> HMSLKSAVKTVLTNSLRSVADGGDWKVLVVDKPALRMISECARMSEILDLGVTVVEDVSKQRKVLPQFHGVYFIEPTEENLDYVIRDFADRTPTYEAAHLFFLSPVPDALMAKLASAKAVKYVKTLKEINTLFIPKEHRVFTLNEPHGLVQYYGSRSSSYNIDHLVRRLSTLCTTMNVAPIVRYSSTSTPGTERMAMQLQKEIDMSVSQGLINAREGKLKSQFLILDRAVDLKSPLVHELTYQAAAYDLLNIENDIYSYSTVDAGGREQQRQVVLGEDDDIWLQMRHLHISEVFRKVKSSFDEFCVSARRLQGLRDSQQGEGGAGALKQMLKDLPQHREQMQKYSLHLDMSNAINMAFSSTIDSCTKAEQNIVTEEEQDGNKVRDFIGEVASVVVDRRVSTEDKLRCLMLCVLAKNGTSSHELNNLLDNANIATPSRSAIYNLEMLGATVVADRRGRKPKTMKRIERDMPYVLSRWTPIVKDLMEYIATGQLDLESYPAVRDGPSVVQPKRASKSVEEDDDGPATSARKRGNWAKNKGNNRSLPSTPSGVAVSGNGAAGAAESAKPKLFVFINGTVSYNEIRCAYEVSQSSGYEVYIGAHNIATPAEFVELVSLLDKADQDVQVLTQGQGDGGLVITTGSAQAGLNLAEV;> MDRLSRLRQMAAENQPAEASDAAGGAEAQIEETSLSAQPEPFMADFFNRVKRIRDNIEDIEQAIEQVAQLHTESLVAVSKEDRDRLNEKLQDTMARISALGNKIRADLKQIEKENKRAQQEGTFEDGTVSTDLRIRQSQHSSLSRKFVKVMTRYNDVQAENKRRYGENVARQCRVVEPSLSDDAIQKVIEHGTEGIFS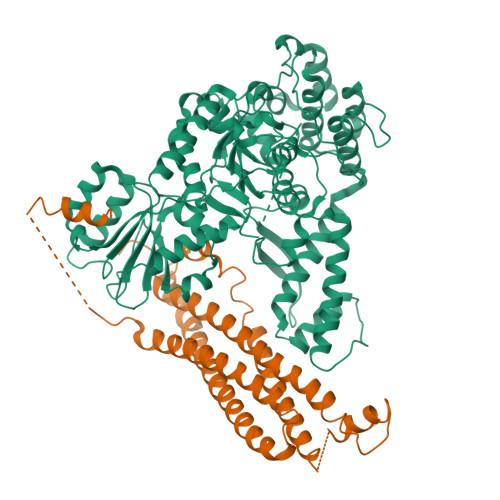GMRLEGAEAKLNEIRDRHKDIQQLERSLLELHEMFTDMSTLVASQGEMIDRIEFSVEQSHNYVKKATEQVVQARHYQESAR>MKDIAIRGYCDRPSVATGETIRFYVSANETRGTFDAELVRLIHGDSNPAGPGYKEEAIKSDLEGQYPARFQRTQFGSYVEVADPDAGLQPDGAFSVHLFLWSTTPSRGRQGIASRWNDERQSGWNLAIEDGRVVFTIGDGSGATSSVVSDRPLFQQIWYSITGVYDPEKKQLRLYQKSVVNRTNSRFGLVVPLDSDCAVSADATVKAADSETSLLIAGLGEAAAQDGRTWCIAHYNGKVDAPKIYGCALGQDDAEKLSRGEIVRPISRLAHWDFSAGIGLNGIPTDHVVDASGYGHHGRCMNQPSRGSTGWNWDGHEENFIHCPEQYGALWFHEDCLDDCRWEKDFEFTVPEGLKSDFYAVKIRYEDTEDYIPFFVLPPRGTATAPILVIASTLSYLAYANEQIMHKADIGQAVAGHTPVLNENDVELHKNLSYYGLSTYDGHIDGRGVQYTSWRRPIMNLRPKHRQGFGSIWELPADLHLIDWLNHNGFEYDVATEHDLNDQGAELLRRYKVVLTGSHPEYQTWANADAWEDYLADGGRGMYLAANGMYWIVEVHPEKPWVMEVRKELGVTAWEAPPGEYHYSTNGRRGGRFRGRARATQKIWGTGMSSFGFDHSGYFVQMPDSQDERVAWIMEGIDPEERIGDGGLVGGGAGGYELDRYDLALGTPPNTLLLASSVEHSVVYTVIPDDKAFPHPGMNGGEHPFVRADITYFSTANGGGMFATSSISWLGSLSWNDYDNNVSKMTKNVLNQFIKDEPAPRVKLAAALEHHHHHH[4x];>[4x]MTEASESCVRDPSNYRDRSADWYAFYDERRRKEIIDIIDEHPEIVEEHAANPFGYRKHPSPYLQRVHNYFRMQPTFGRYYIYSEREWDAYRIATIREFGELPELGDERFKTEEEAMHAVFLRRIEDVRAELA

Certain bacterial species from genera such as Paracoccus, Pseudomonas, and Alcaligenes have evolved to use DMF as a sole carbon and nitrogen source for growth via degradation by a dimethylformamidase (DMFase). We show that DMFase from Paracoccus sp. strain DMF is a halophilic and thermostable enzyme comprising a multimeric complex of the α2β2 or (α2β2)2 type. The active site consists of a mononuclear iron coordinated by two Tyr side‐chain phenolates and one carboxylate from Glu. The Fe3+ ion in the active site catalyzes the hydrolytic cleavage of the amide bond in DMF.

When the purified native or recombinant parDMFase was imaged on ice by electron cryo‐microscopy (cryoEM), the micrographs unambiguously revealed two populations: a smaller molecule measuring approximately 100 Å diameter and a larger structure of approximately 150 Å in diameter could be identified. Subsequent 2D classification showed that the smaller unit was a dimer, and the larger structure was a dimer of dimers. The dimer of dimers (called tetramer here) has a total mass of 400 kDa. We noted that the salt concentration in the buffer shifts the oligomer (dimer/tetramer) equilibrium. In the presence of low salt, the enzyme is predominantly in the dimeric form, and this equilibrium shifted to the tetramer at higher salt concentrations (≥200 mm). Subsequently, we collected two data sets with no salt and 200 mm NaCl yielding reconstructions with an overall resolution of 3 Å (dimer) and 2.8 Å (tetramer), respectively. The local resolution plot of both maps showed that much of the reconstruction was resolved between 2.5–3.5 Å. The high quality of the maps allowed de novo tracing of polypeptide chains of both the large and small subunits. We used the dimer map for the initial tracing, and the final model is shown in Figure 2 B. The model from the dimer was used to obtain the tetramer model. The mononuclear Fe atom is tetra‐coordinated with the protein. It is coordinated to two phenolates of tyrosine residues (Y399 and Y440 serve as monodentate ligands), and a glutamic acid carboxylate side chain (E521 serves as a bidentate ligand).>[10x]MGSSHHHHHHSSGLVPRGSPTYVGKEA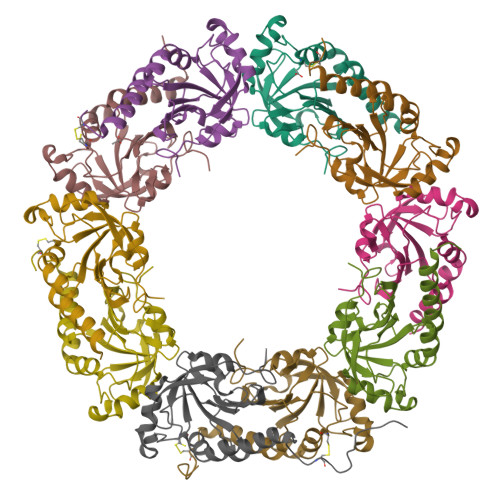PFFKAEAVFGDNSFGEVNLTQFIGKKYVLLYFYPLDFTFVCPSEIIALDKALDAFHERNVELLGCSVDSKYTHLAWKKTPLAKGGIGNIKHTLLSDITKSISKDYNVLFDDSVSLRAFVLIDMNGIVQHLLVNNLAIGRSVDEILRIIDAIQHHEKYGDVCPANWQKGKVSMKPSEEGVAQYLSTL In the present study, a vaccine antigen based on the fusion of two known NTHi adhesive proteins, protein E (PE) and a pilin subunit (PilA), was developed. PE is a ubiquitous NTHi antigen described to be important for the adhesion of the bacterium to epithelial cells. It is also known to bind vitronectin, which protects the bacterium from complement attack, and immunization with a fragment of PE was shown to afford protection in a mouse model of pulmonary clearance. PilA is another ubiquitous NTHi antigen described to be a conserved protein among H. influenzae isolates. It is the major subunit of type IV pili (Tfp), which are hair-like filaments involved in adherence through ICAM-1 (25).

PE crystallized in space group C2 with a monomer in the asymmetric unit, but crystal packing revealed a head-to-tail dimer on the crystallographic 2-fold axis that had an interface area of approximately 950 Å2, as determined by the software Protein Interfaces, Surfaces and Assemblies (PISA) run within the COOT model-building tool. The PE monomer comprises a β-sheet with six antiparallel β-strands and two C-terminal α-helices, with one of these being formed by heterologous amino acids added in the PE construct used for the crystallization. A disulfide bond exists between Cys81 and Cys130, linking the main α-helix with the end of β4, which confirms the mass spectrometry data (see below). The PE crystal structure is comparable to the published structure, as revealed by their superposition. The recently published crystal structure of PE showed a noncrystallographic symmetry dimer that the authors suggest is the dimer observed in solution, despite the relatively low interface area (∼625 Å2). It was the largest interface in their crystal system, but this type of dimer has not been observed in our crystal systems. The contrasting types of PE dimers observed may simply be due to differences in crystallization conditions.

> QIQKAEQNDVKLAPPTDVRSGYIRLVKNVNYYIDSESIWVDNQEPQIVHFDAVVNLDKGLYVYPEPKRYARSVRQYKILNCANYHLTQVRTDFYDEFWGQGLRAAPKKQKKHTLSLTPDTTLYNAAQIICANYGEAFSVDKKKLAAALEHHHHHH>[2x]RSPWARW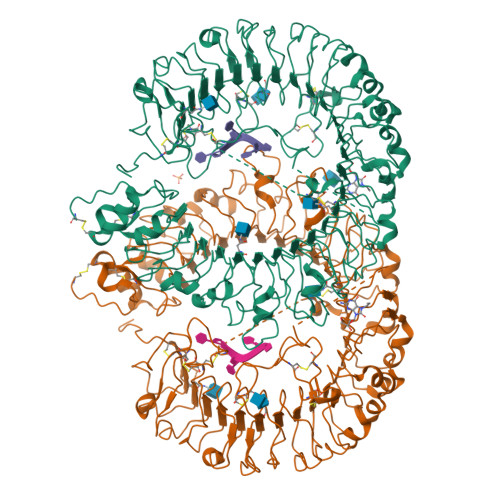FPKTLPCDVTLDVSKNHVIVDCTDKHLTEIPGGIPTNTTNLTLTINHIPDISPASFHRLVHLVEIDFRCNCVPIRLGSKSNMCPRRLQIKPRSFSGLTYLKSLYLDGNQLLEIPQGLPPSLQLLSLEANNIFSIRKEQLTELANIEILYLGQNCYYRNPCYVSYSIEKDAFLNLTKLKVLSLKDNNVTTVPTVLPSTLTELYLYNNMIAEIQEDDFNNLNQLQILDLSGNCPRCYNAPFPCTPCKNNSPLQIPVNAFDALTELKVLRLHSNSLQHVPPRWFKNINNLQELDLSQNFLAKEIGDAKFLHFLPNLIQLDLSFNFELQVYRASMNLSQAFSSLKSLKILRIRGYVFKELKSFQLSPLHNLQNLEVLDLGTNFIKIANLSMFKQFKRLKVIDLSVNKISPSGDSSEVGFCSNARTSVESYEPQVLEQLYYFRYDKYARSCRFKNKEASFTSVQESCYKYGQTLDLSKNSIFFIKSSDFQHLSFLKCLNLSGNLISQTLNGSEFQPLAELRYLDFSNNRLDLLHSTAFEELRKLEVLDISSNSHYFQSEGITHMLNFTKNLKVLQKLMMNDNDISSSTSRTMESESLRTLEFRGNHLDVLWRDGDNRYLQLFKNLLKLEELDISKNSLSFLPSGVFDGMPPNLKNLSLAKNGLKSFIWEKLRYLKNLETLDLSHNQLTTVPERLSNCSRSLKNLILKNNQIRSLTKYFLQDAFQLRYLDLSSNKIQMIQKTSFPENVLNNLKMLLLHHNRFLCTCDAVWFVWWVQHTEVTIPYLATDVTCVGPGAHKGQSVISLDLYTCELDLTN>[2x]MLQNSFKLAQSLRNGFYRNAWRAFSSHGPRQPLVSPERRLEKAHPTFTERSQLKYARRLVVKLGSAVITREDNHGLALGRLASIVEQVAECHLEGREVMMVTSGAVAFGKQKLAQELLMSLSMRETLNPKDSKEFDGATLEPRAAAAVGQSGLMSLYDAMFAQYGVKIAQVLVTKPDFYNEETRNNLFCTLSELISLNIVPIINTNDAVSPPMFIRDDEPAGGARRGIPIKDNDSLSAMLAAEVQADLLILMSDVDGIYNKPPWEDGAKLMHTYTSDDSNSIEFGKKSK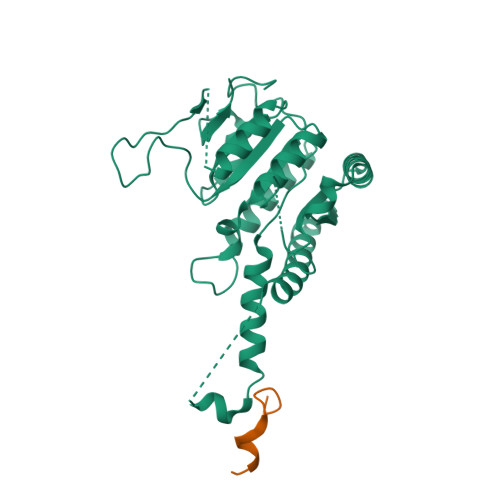VGTGGMDSKVKAATWALDRGVSVVICNGMQEKAIKTIIGGRKVGTFFTEATESANAVPVEVMAENARTGSRQMQALTPAQRASAVNTLADLLVSREKFILDANAKDLAEAQKSGLAKPLLSRLSLNPAKLKNLSVGLKQIAEDSHKNVGRVLRRTRLADQLELKQVTVPIGVLLVIFESRPDSLPQVAALAMASANGLLLKGGKEAAHSNKALMELVKEALATVGAEHAVSLVSTREEISDLLSMENHIDLIIPRGSSDLVRSIQQQSLHIPVLGHAEGVCHVYIDRDADLEKALRIARDAKCDYPAACNAMETLLIHEDLMSGAIFGDVCNMLKREGVKIYAGPRLNQQLTFGPPAAKSLKHEYGALECCIEVVPSLDEAINHIHTYGSSHTDVIVTENDAAARQFLGSVDSACVFHNASSRFADGFRFGLGAEVGISTARIHARGPVGVEGLLTTKWILEGQDHAAADFAEGGGRTWLHETLPLD> SMSVKKPKRDDSKDLALCSMILTEMETHEDAWPFLLPVNLKLVPGYKKVIKKPMDFSTIREKLSSGQYPNLETFALDVRLVFDNCE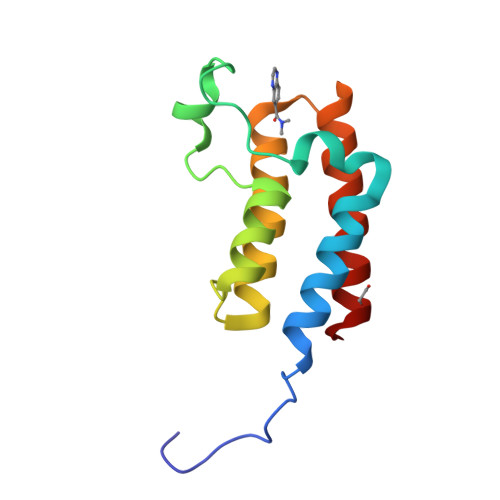TFNEDDSDIGRAGHNMRKYFEKKWTDTFK>MHPQTLEQIKESESQLSGRVGMVELDLASGRTLSYRADERFPMMSTFKVLLCGAVLARVDAGLEQLDRRIHYRQQDLVEYSPVTEKHLADGMTVAELCAAAITMSDNTAANLLLAT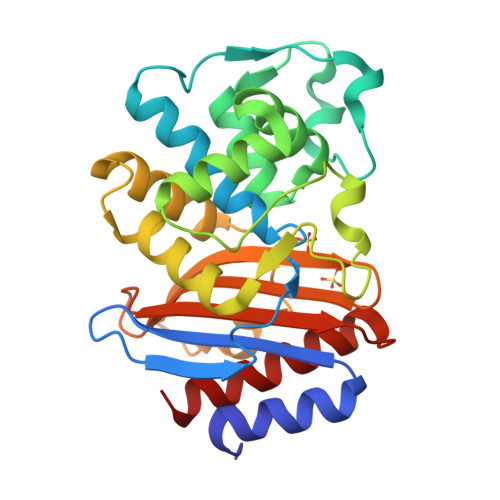IGGPAGLTAFLRNIGDNVTRLDRWETELNEALPGDERDTTTPAAMAATLRKLLTGEILSAASRQQLITWMVADKVAGPLLRSVLPAGWFIADKTGAGERGSRGIIAVLGPDGKPSRIVVIYLTETQASMDERNQQIAEIGAALIEHW[2x]>GHMNDLIDTTEMYLRTIYDLEEEGVVPLRARIAERLEQSGPTVSQTVARMERDGLLTVAEDRHLELTKAGRARAISVMRKHRLAERLLVDVIGLEWEQVHLEACRWEHVMSEAVERKLVKLLGNPTTSPYGNPIPGLDELGVGDSVEPVDTDLRRVDEVARSGGGRALVCRIAEHVQLDPDLMSELKKVGVVPGNEID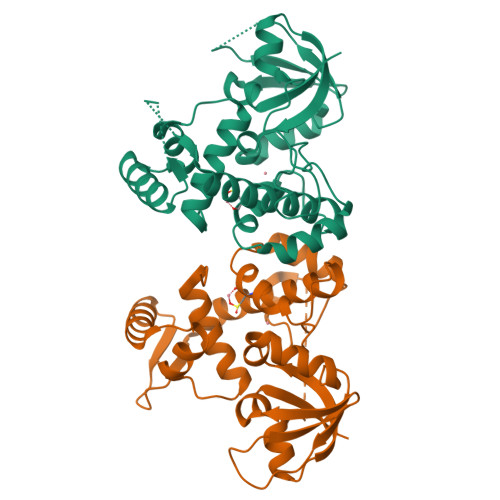IVAVAGVNKPIQVQGSEGGTQLQPGIAHAVMVRVK[2x]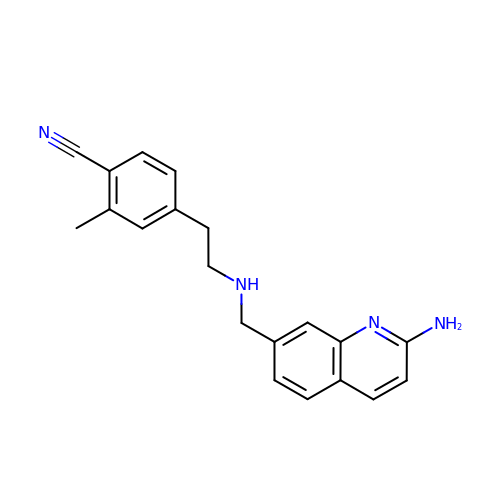4-(2-{[(2-aminoquinolin-7-yl)methyl]amino}ethyl)-2-methylbenzonitrile | C20 H20 N4 | OFELXUWNGBXCPK-UHFFFAOYSA-N> AYTFDSTMLDTNSGESIDVSLFNQGLQLPGNYFVNVFVNGRKVDSGNIDFRLEKHNGKELLWPCLSSLQLTKYGIDIDKYPDLIKSGTE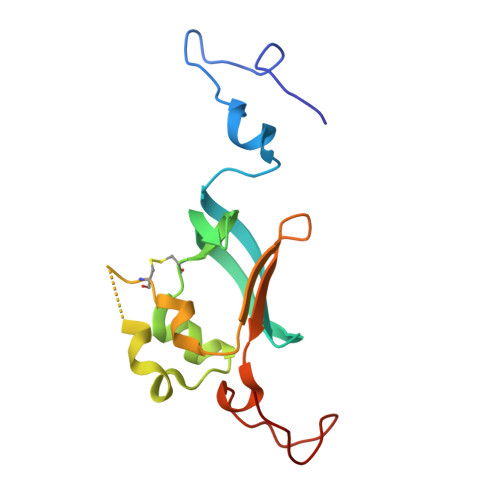QCVDLLAIPHSDVQFYFNQQKLSLIVPPQALLPRFDGIMPMQLWDDG>MSVIKPEMKIKLRMEGAVNGHKFVIEGEGIGKPYEGTQTLDLTVKEGAPLPFSYDILTPAFQYGNRAFTKYPKDIPDYFKQAFPEGYSWERSMTYEDQGICIATSDITMEGDCFFYKIRFDGTNFPPNGPVMQKKTLKWE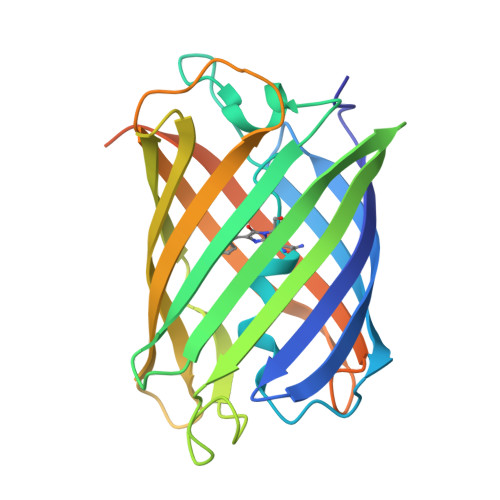PSTEKMYVRDGVLKGDVNMALLLEGGGHYRCDFKTTYKAKKDVRLPDAHEVDQRIEILSHDKDYNKVRLYEHAEARYSMLPSQAKASGKPIPNPLLGLDSTHHHHHH[4x]>[2x]MFLRIDRLQIELPMPKEQDPNAAAAVQA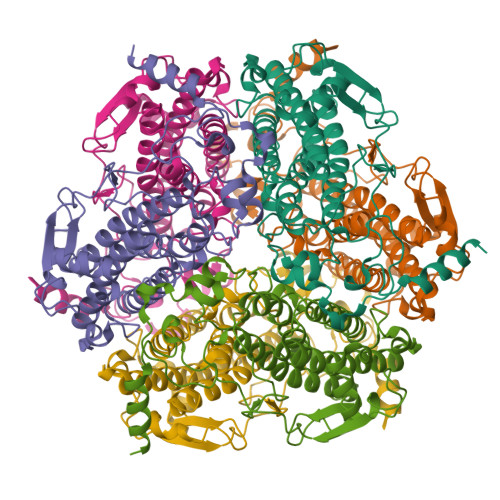LLGGRFGEMSTLMNYMYQSFNFRGKKALKPYYDLIANIATEELGHIELVAATINSLLAKNPGKDLEEGVDPESAPLGFAKDVRNAAHFIAGGANSLVMGAMGEHWNGEYVFTSGNLILDLLHNFFLEVAARTHKLRVYEMTDNPVAREMIGYLLVRGGVHAAAYGKALESLTGVEMTKMLPIPKIDNSKIPEAKKYMDLGFHRNLYRFSPEDYRDLGLIWKGASPEDGTEVVVVDGPPTGGPVFDAGHDAAEFAPEFHPGELYEIAKKLYEKAK> MGHHHHHHMKPYYVTTAIAYPNAAPHVGHAYEYIATDAIARFKRLDRYDVRFLTGTDEHGLKVAQAAAAAGVPTAALARRNSDVFQRMQEALNISFDRFIRTTDADHHEASKELWRRMSAAGDIYLDNYSGWYSVRDERFFVESETQLVDGT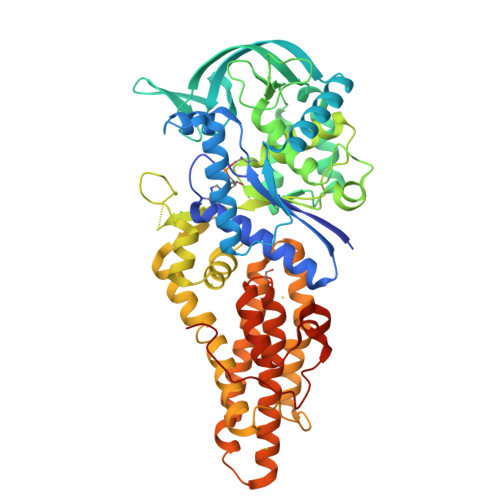RLTVETGTPVTWTEEQTYFFRLSAYTDKLLAHYHANPDFIAPETRRNEVISFVSGGLDDLSISRTSFDWGVQVPEHPDHVMYVWVDALTNYLTGAGFPDTDSELFRRYWPADLHMIGKDIIRFHAVYWPAFLMSAGIELPRRIFAHGFLHNRGEKMSKSVGNIVDPVALAEALGVDQVRYFLLREVPFGQDGSYSDEAIVTRINTDLANELGNLAQRSLSMVAKNLDGRVPNPGEFADADAALLATADGLLERVRGHFDAQAMHLALEAIWLMLGDANKYFSVQQPWVLRKSESEADQARFRTTLYVTCEVVRIAALLIQPVMPESAGKILDLLGQAPNQRSFAAVGVRLTPGTALPPPTGVFPRYQPPQPPEGKRS> MPSELTPEERSELKNSIAEFHTYQLDPGSCSSLHAQRIHAPPELVWSIVRRFDKPQTYRHFIKSCSVEQNFEMRVGCTR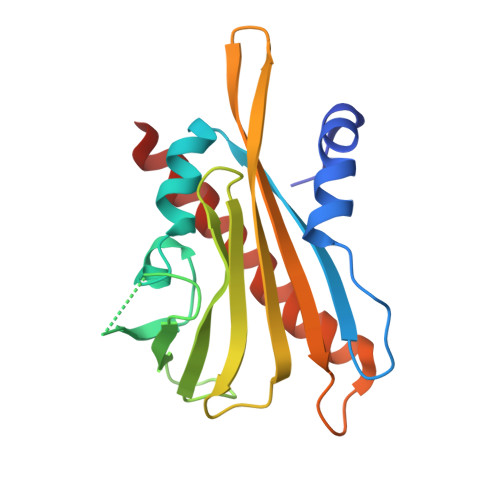DIIVISGLPANTSTERLDILDDERRVTGASIIGGEHRLTNYKSVTTVHRFEKENRIWTVVLESYVVDMPEGNSEDDTRMLADTVVKLNLQKLATVAEAMARN> SLFEQLGGQAAVQAVTAQFYANIQADATVATFFNGIDMPNQTNKTAAFLCAALGGPNAWTGRNL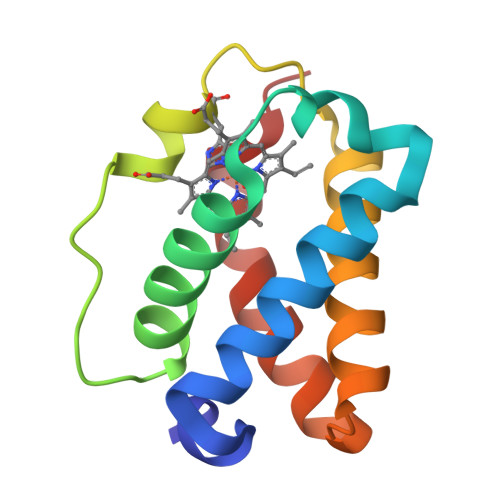KEVHANMGVSNAQFTTVIGHLRSALTGAGVAAALVEQTVAVAETVRGDVVTV2-chloranyl-4-nitro-phenol | C6 H4 Cl N O3 | 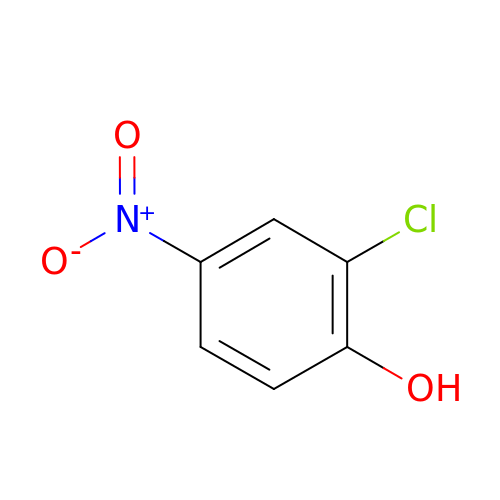BOFRXDMCQRTGII-UHFFFAOYSA-N4-azanyl-7-(1-methylcyclopropyl)-~{N}-(5-methyl-1~{H}-pyrazol-3-yl)pyrrolo[2,3-d]pyrimidine-5-carboxamide | C15 H17 N7 O | 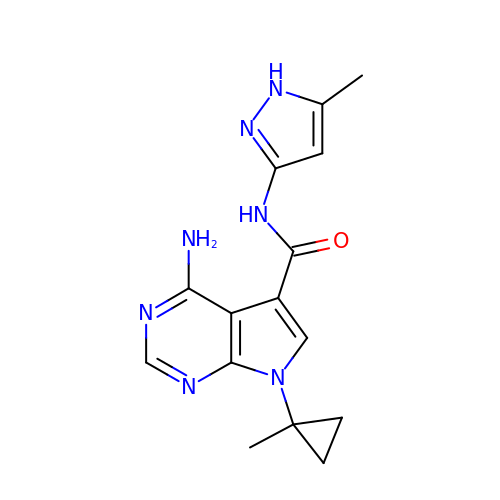VKNSWNWSJODLGL-UHFFFAOYSA-N> MTKLFSKVKESIEGIKMPSTLTINGKAPIVAYAELIAARIVNALAPNSIAIKLVDDKKAPAAKLDDATEDVFNKITSKFAAIFDNGDKEQVAKWVNLAQKELVIKNFAKLSQSLETLDSQLNLRTFILGGLKYSAADVAC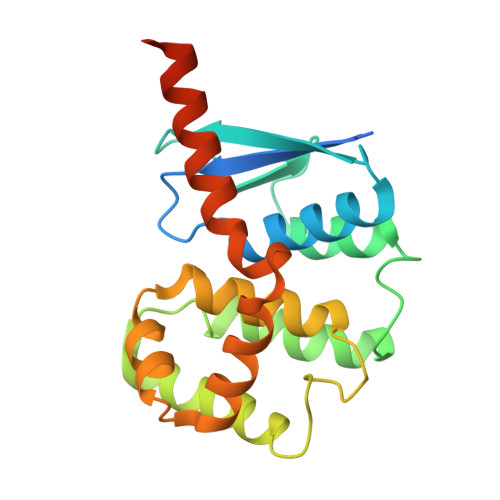WGALRSNGMCGSIIKNKVDVNVSRWYTLLEMDPIFGEAHDFLSKSLLELKKSANVGKKKETHKANFE Dye-decolourising peroxidases (DyPs) are a distinct structural family of peroxidases possessing an α + β dimeric fold that houses a b-type heme coordinated on its proximal side by a His residue. The soil dwelling bacterium, Streptomyces lividans possesses three DyPs; two belonging to the A-type and a third belonging to the B-type sub-families. The two A-type homologs, named DtpA and DtpAa react in their ferric heme state with H2O2 to form a two-electron oxidised derivative that is an Fe(iv)O heme carrying a porphyrin π-cation radical (Fe(iv)O[Por˙+]) – termed compound I.34–36 In the presence of a substrate, reduction of the porphyrin π-cation radical results in the formation of compound II (Fe(iv)O), with a second substrate molecule reducing compound II to the ferric state. By using an A-type member of the DyP family (DtpAa) as an exemplar, we combine protein engineering, X-ray crystallography, hole-hopping calculations, EPR spectroscopy and kinetic modelling to provide compelling new insights into the control of radical migration pathways following reaction of the heme with hydrogen peroxide.

The Y345F variant, creates a DtpAa protein with no Tyr residues within 15 Å of the heme on the distal side with the double variant, Y345F/F347Y, mimicking the distal heme Tyr arrangement as in DtpA. High-resolution X-ray crystal structures determined to 1.23 Å (Y345F) and 1.27 Å (Y345F/F347) resolutions, corroborated the desired amino acid changes. Not surprisingly, the fastest hole hopping pathways (τM 10−3 s) in the Y345F and double variant remain dominated by the proximal Trp/Tyr dyad.

>[2x]MTDTDSPAPAPSPSRRSLIGWGGAGLALGAAAAAGGAVAMDRAGADADPAGADAGSAVPFHGAHQAGIATPVQDRLHFAAFDVTTEDRAAFVALLKEWTAAARRLTAGHAVGEGAYGGLPEAPPDDTGEALGLKPSRLTLTIGFGPSLFTRFGLADLRPEALADLPKFPGDNLDRARSGGDLCVQACADDPQVAVHAIRNLARIGFGKVVVRWSQLGFGKTSSTTPDKQTPRNLLGFKDGTRNIAGTEKDRLDRFVWAAEKDGTPWMTGGSYLVARRIRMHIETWDRASLQEQEDVFGRDKGEGAPVGKAKERDEPFLKAMKPDAHVRLAHPDSNGGATLLRRGFSFTDGTDGLGRLDAGLFFLAYQRDIRTGFVPVQRNLATDALNEYIQHVGSAVFAVPPGVRDADDWWGSTLFG[azanyl-[(2E)-2-(1-phenylethylidene)hydrazinyl]methylidene]azanium | C9 H13 N4 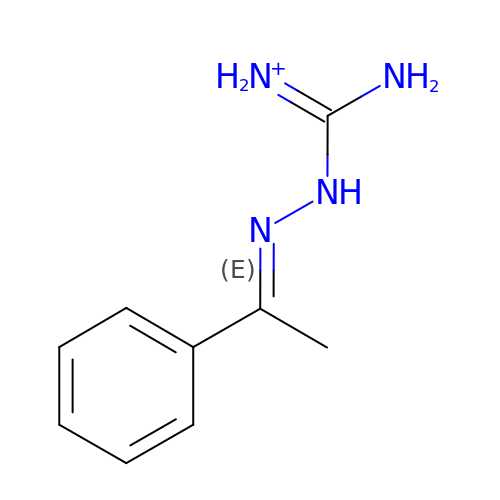| MRKZNCISKCWGLP-KPKJPENVSA-O>[2x]P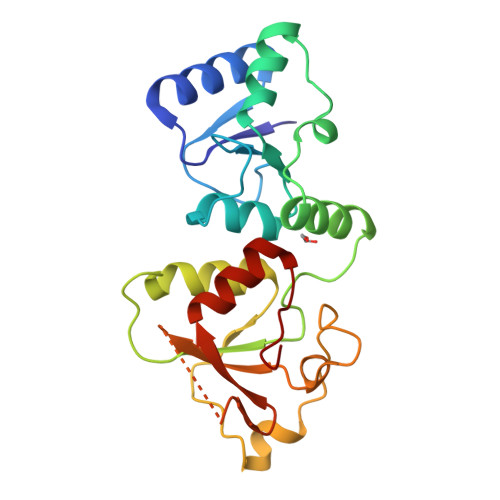LVLIGSGLSSEQQKMLSELAVILKAKKYTEFDSTVTHVVVPGDAVQSTLKCMLGILNGCWILKFEWVKACLRRKVCEQEEKYEIPEGPRRSRLNREQLLPKLFDGCYFYLWGTFKHHPKDNLIKLVTAGGGQILSRKPKPDSDVTQTINTVAYHARPDSDQRFCTQYIIYEDLCNYHPERVRQGKVWKAPSSWFIDCVMSFELLPLDS>[4x]MAKIKNPILTGFHPDPSICRVGDDYYIAVSTFEWFPGVRIYHSKDLKNWRLVARPLNRLSQLNMIGNPDSGGVWAPHLSYSDGKFWLIYTDVKVVEGQWKDGHNYLVTCDTIDGAWSDPIYLNSSGFGPSL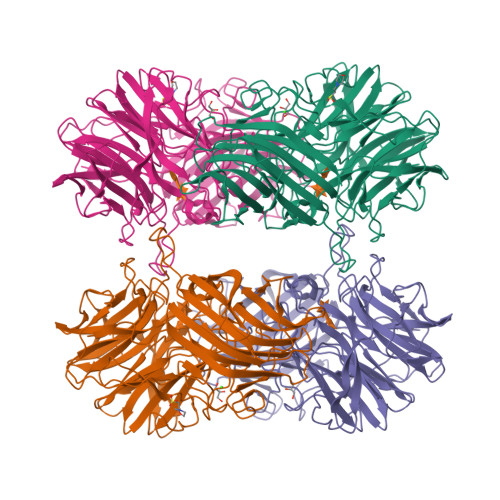FHDEDGRKYLVNMYWDHRVDHHPFYGIVLQEYSVEQKKLVGEPKIIFKGTDLRITEGPHLYKINGYYYLLTAEGGTRYNHAATIARSTSLYGPYEVHPDNPLLTSWPYPRNPLQKAGHASIVHTHTDEWFLVHLTGRPLPREGQPLLEHRGYCPLGRETAIQRLEWKDGWPYVVGGNGPSLEIDGPSVEEVSWEKDYDEKDDFDGDTLNHHFQTLRIPLGEDIATLKARPGHLRLYGRESLTSRFTQAFVARRWQHFHFVAETKVSFRPTTFQQSAGLVNYYNTQNWTTLQITWHEEKGRILELMTCDHLVVDQPLRGREIVVPDDIEYVYLRVTVQATTYKYSYSFDGMNWIDLPVTFESYKLSDDYIKSRAAFTGAFVGMHCRDGSGQNNYADFDYFLYKEL>[3x]MLNPIVRKFQYGQHTVTLETGMMARQATAAVMVSMDDTAVFVTVVGQKKAKPGQDFFPLTVNYQERTYAAGRIPGSFFRREGRPSEGETLIARLIDRPIRPLFPEGFVNEVQVIATVVSVNPQVNPDIVAMIGASAALSLSGIPFNGPIGAARVGYINDQYVLNPTQDELKESKLD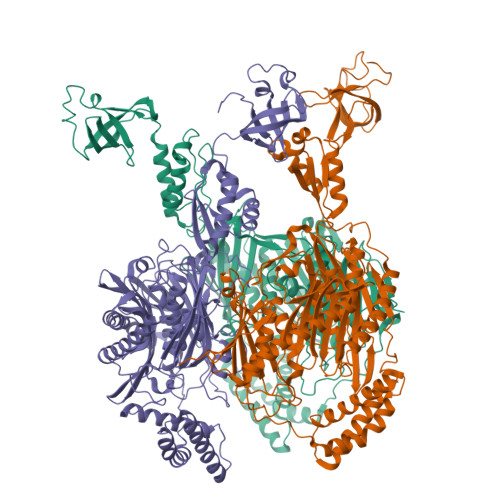LVVAGTEAAVLMVESEAQLLSEDQMLGAVVFGHEQQQVVIQNINELVKEAGKPRWDWQPEPVNEALNARVAALAEARLSDAYRITDKQERYAQVDVIKSETIATLLAEDETLDENELGEILHAIEKNVVRSRVLAGEPRIDGREKDMIRGLDVRTGVLPRTHGSALFTRGETQALVTATLGTARDAQVLDELMGERTDTFLFHYNFPPYSVGETGMVGSPKRREIGHGRLAKRGVLAVMPDMDKFPYTVRVVSEITESNGSSSMASVCGASLALMDAGVPIKAAVAGIAMGLVKEGDNYVVLSDILGDEDHLGDMDFKVAGSRDGISALQMDIKIEGITKEIMQVALNQAKGARLHILGVMEQAINAPRGDISEFAPRIHTIKINPDKIKDVIGKGGSVIRALTEETGTTIEIEDDGTVKIAATDGEKAKHAIRRIEEITAEIEVGRVYTGKVTRIVDFGAFVAIGGGKEGLVHISQIADKRVEKVTDYLQMGQEVPVKVLEVDRQGRIRLSIKEATEQSQPAAAPEAPAAEQGE> NLSELDRLLLELNAVQHNPP;> SGRHERDAFDTLFDHAPDKLNVVKKTLITFVNKHLNKLNLEVTELETQFADGVYLVLLMGLLEGYFVPLHSFFLTPDSFEQKVLNVSFA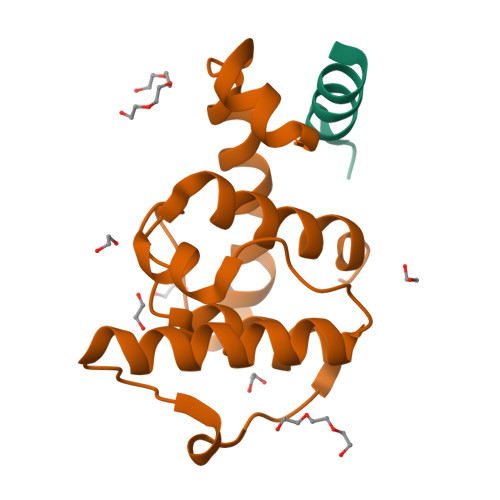FELMQDGGLEKPKPRPEDIVNCDLKSTLRVLYNLFTKYRNVE South-methanocarba-2'-deoxyadenosine triphosphate | C12 H18 N5 O11 P3 | 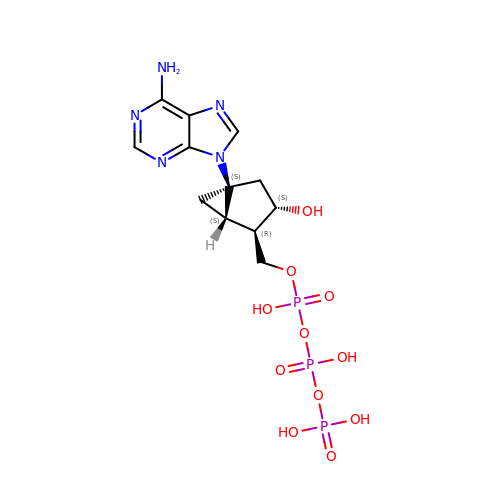DNBZILMJAUSGHT-QZOVBDONSA-N>[4x]MADEIAKAQVARPGGDTIFGKIIRKEIPAKIIFEDDRCLAFHDISPQAPTHFLVIPKKHI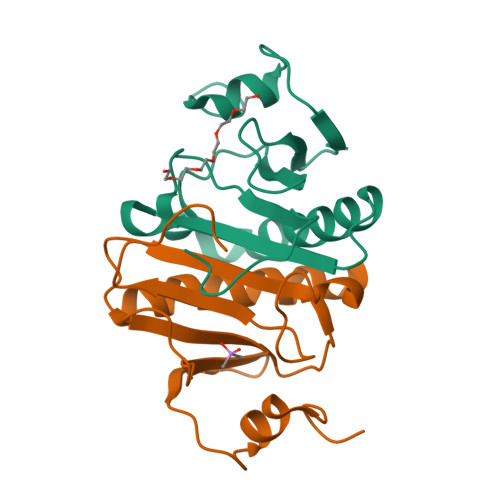SAISVAEDDDESLLGHLMIVGKKCAADLGLNKGYRMVVNEGSDGGQSVYHVHLHVLGGRQMHWPPG2-{(R)-(2-chlorophenyl)[2-(piperidin-1-yl)ethoxy]methyl}-1H-pyrrolo[3,2-b]pyridine-7-carboxylic acid | C22 H24 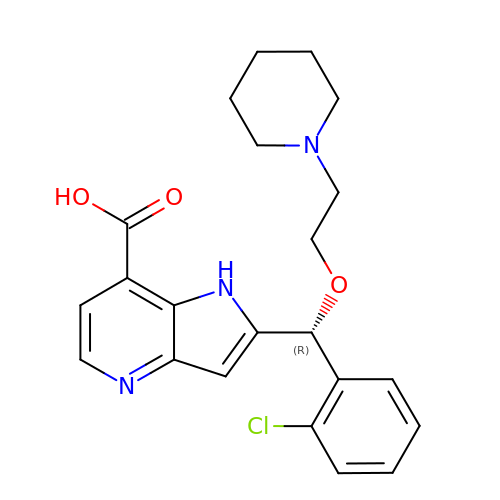Cl N3 O3 | AWPYWZMMJZGPOX-OAQYLSRUSA-N4-bromobenzoic acid | C7 H5 Br O2 | 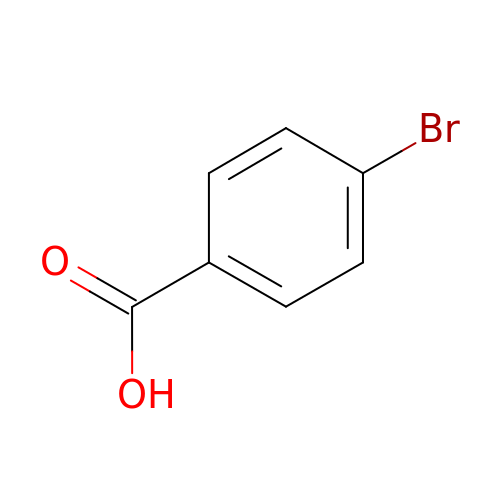TUXYZHVUPGXXQG-UHFFFAOYSA-N>MKTKEDMQELYFPTPKLIEWENGVRQYSTVRGDTEVLMSYVPPHTNVEPHQHKEVQIGMVVSGELMMTVGDVTRKMTALESAYIAPPHVPHGARNDTDQEVIAIDIKRLKADETYTSPEDYFLDIFKTRDLLPGMEVTFFVEDWVEIMLAKIPGNGGEMPFHKHRNEQIGICIGGGYDMTVEGCTVEMKFGTAYFCEPREDHGA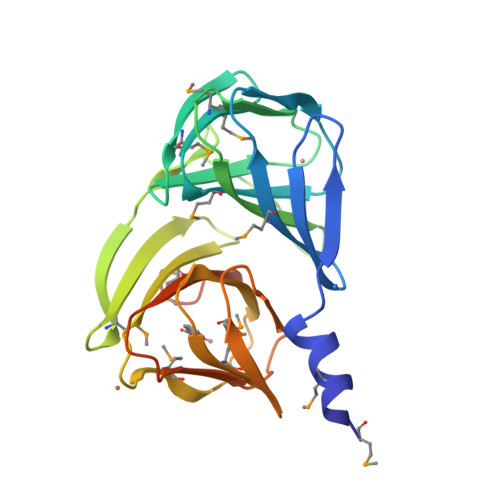INRSEKESKSINIFFPPRYNRAKAKKMKADELEHHHHHH[2x]> AQAFVNSKIQPGKVVVFIKPTCPFCRKTQELLSQLPFKEGLLEFVDITATSDTNEIQDYLQQLTGARTVPRVFIGKECIGGCTDLES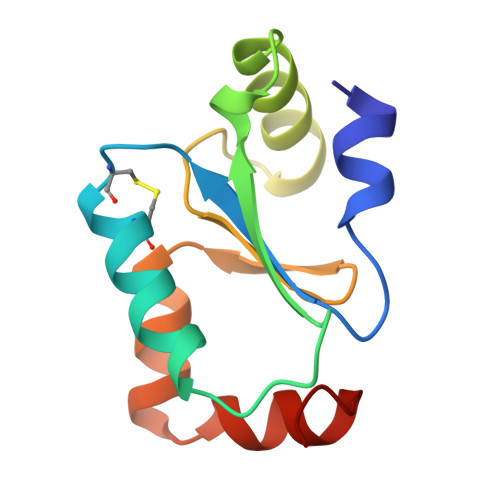MHKRGELLTRLQQVGAVK> ALHPMTKVIFNGLDVNTEVQPLSDDFKQISDPKGYLTYSVKYEDQFTKKDKLRASEADDRIVGPTVNLFKYGAAVVNIDLNRDFFDTATGIDLTKGIPLVQDLLVPIGVTAGAEQSAEYVSGLLMVLFKVMTDNRLVIVGETTTPMSNTLSTVVNNVLRTTYHNNVGVNPALLRDFTQVNWLNRDITNMLQQAGTKYGLGLTETRLDYVRLVKTIVGHALNIDHFAASVLNINLRALMEANVTADDRIKALQAHSMISTQFHGPNQG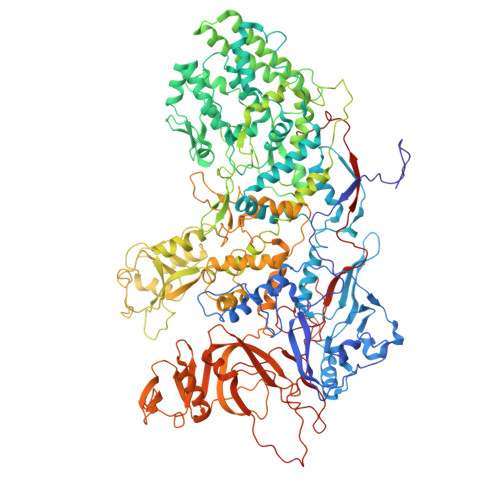ALRPELAFDHDHIIRCLMLAAANYPRLEGIIVQINTGYVASANVIRPVSEKRYFPENLEQNQSAARLVSAVKARASEADISSIHLAIAREVSPMFNVHELKKIAESFEDPSSIVVVLEFILFALFFPTEFNRIKGDIQNVLLLFFSRWYPVEYGIFIQRGATYTINAAGEFEFSGRNEKWDQSLYLSEHFPALFSDVPLAGANTIIAIMRLFTPQGFLRTDDLAIAANFPRASRNPQTYIPYTNQRGTVTNEFASRFRTIVATLANVVNERAVQDDMQKATRSCTKQWLRHLETQFDNIAVAHTDHLSVVYATMSNFMLNFTNNFSGNHATFKPDQYVITSPEGSYKPIIERQGETVDGLTIIDTSIVWPILCQCTYPLVRQSGKGVDAVSIMEEIVYPDPSTTLSQSLSVAQVLSKLTLPDAFINMILSGGDSVVMRTYQTEADDDLDEGIRMTTYDQYLSHIRERLHITNVPDPIYITGASTPDQIAASVQATHVAVVLYQSGVINGSASTYLRENEVLVVMPDYYDVVSRFANANLQMNNNRYHESVLEIADIFDQADFIQTSDAVRQLRALMPTLSTSQIRHAIERIAQITDVDSTDYGKLTLRFLGTLTRSLKMQNAQIRRIRPDGTVLRYDDQIDIEAFRWSRYFLDELRLRRLSVGLRLITNPRIARRFDGVRIMYLTDDDPDPDFVPDVPEGYVAVQYAHRLFSSSLANKRNRVTYTHPPTGMAYPSPTGRPHVHMTINERAGMSKLVADNIIASVIKSNWVVDIHDIEYTAEVMTPSEGYTQHVDAESIMTAPKGKLFHLQFMDGLLRPEPSAFDPPASGEDMRLIYPLQPISVARSMRAIVNHNEVDRPRGAVAPSSYEMDTGTLSRNGDLLYSPVANGQVGIPKLEVDHISFSNVVSMMTANIRTGDDMAVERVNPDDVRAINIRNA>MMVISEKVRKALNDQLNREIYSSYLYLSMATYFDAEGFKEFAHWMKKQ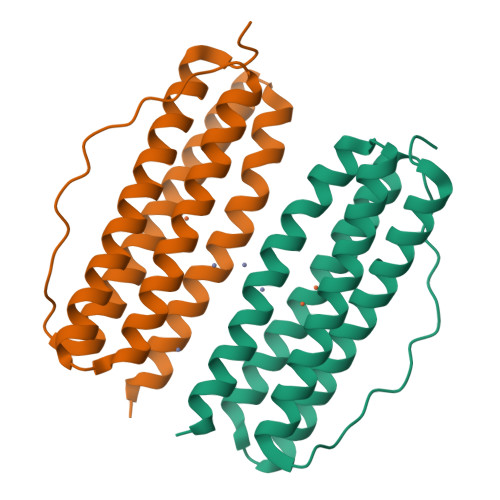AQEELTHAMKFYEYIYERGGRVELEAIEKPPSNWNGIKDAFEAALKHEEFVTQSIYNILELASEEKDHATVSFLKWFVDEQVEEEDQVREILDLLEKANG[2x]> MSAKAAPKTLHQVRNVAYFFAAWLGVQKGYIEKS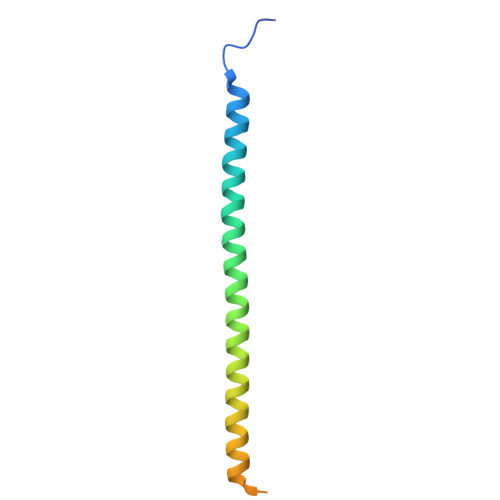ANDRLWVEHQRKVRQQNVERQQALDSIKLMQQGVRATTPGQLEGVPAELQQLAEAFTK> MHHHHHHDDDDKRT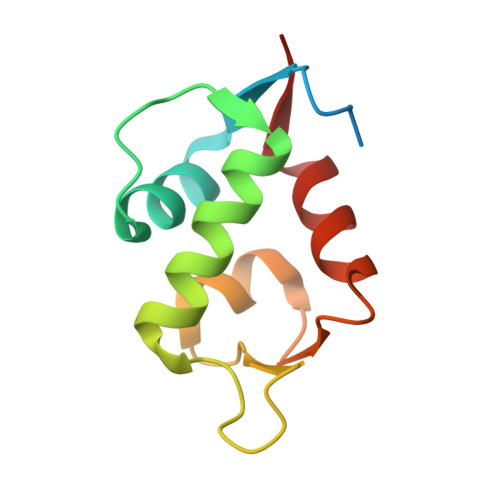LPGEGTQVHPRAPLLQILKVAGAQEEVFTVKEVMHYLGQYIMMKQLYDKQRQHIVHCHDDPLGELLEVGSFSVKNPSPLYEMLKRNLVIL>MKLDIKKTFSNRSDRVKGIDFHPTEPWVLTTLYSGRVEIWNYETQVEVRSIQVTETPVRAGKFIARKNWIIVGSDDFRIRVFNYNTGEKVVDFEAHPDYIRSIAVHPTKPYVLSGSDD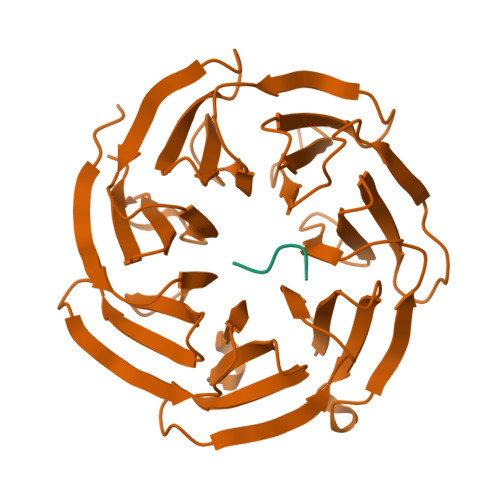LTVKLWNWENNWALEQTFEGHEHFVMCVAFNPKDPSTFASGCLDRTVKVWSLGQSTPNFTLTTGQERGVNYVDYYPLPDKPYMITASDDLTIKIWDYQTKSCVATLEGHMSNVSFAVFHPTLPIIISGSEDGTLKIWNSSTYKVEKTLNVGLERSWCIATHPTGRKNYIASGFDNGFTVLSLG[2x];>[2x]AKEKSD> MAILGLGTDIVEIARIEAVIA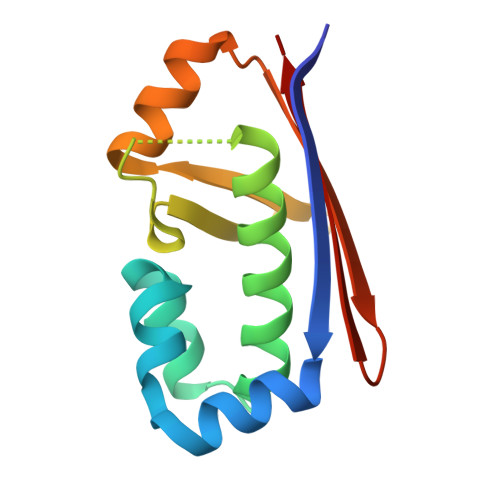RSGDRLARRVLSDNEWAIWKTHHQPVRFLAKRFAVKEAAAKAFGTGIRNGLAFNQFEVFNDELGKPRLRLWGEALKLAEKLGVANMHVTLADERHYACATVIIES> MSE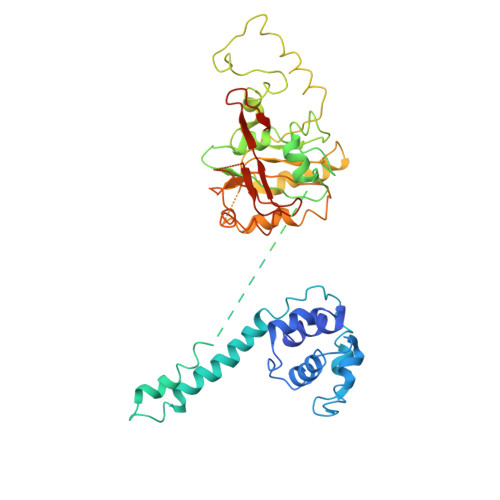LFSERIPPQSIEAEQAVLGAVFLDPAALVPASEILIPEDFYRAAHQKIFHAMLRVADRGEPVDLVTVTAELAASEQLEEIGGVSYLSELADAVPTAANVEYYARIVEEKSVLRRLIRTATSIAQDGYTREDEIDVLLDEADRKIMEVSQRKHSGAFKNIKDILVQTYDNIEMLHNRDGEITGIPTGFTELDRMTSGFQRSDLIIVAARPSVGKTAFALNIAQNVATKTNENVAIFSLEMSAQQLVMRMLCAEGNINAQNLRTGKLTPEDWGKLTMAMGSLSNAGIYIDDTPSIRVSDIRAKCRRLKQESGLGMIVIDYLQLIQGSGRSKENRQQEVSEISRSLKALARELEVPVIALSQLSRSVEQRQDKRPMMSDIRESGSIEQDADIVAFLYRDDYYNKDSENKNIIEIIIAKQRNGPVGTVQLAFIKEYNKFVNLERRFDEAQIPPGA>GSHMKNSVSVDLPGSMKVLVSKSSNADGKYDLIATVDALELSGTSDKNNGSGVLEGVKADASKVKLTISDDLGQTTLEVFKSDGSTLVSKKVTSKDKSSTYELFNEKGELSFKYITRADKSSTYELFNEKGELSFKYITRADKSSTYELFNEKGELSFKYITRADKSSTYELFNEKGELSFKYITRADGTRLEYTGIKSDGSGKAKEVLKGYVLEGTLTAEKTTLVVKEGTVTLSKNISKSGEVSVELNDTDSSAAT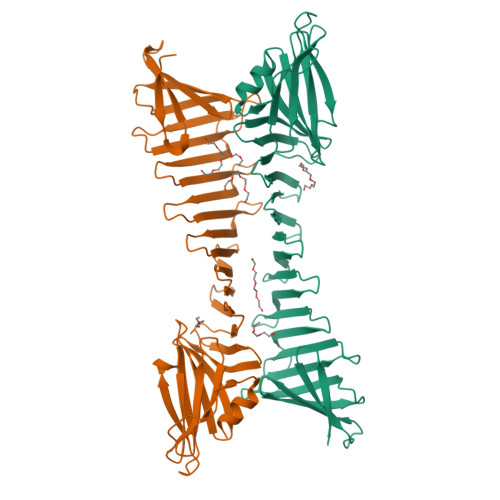KKTAAWNSGTSTLTITVNSKKTKDLVFTSSNTITVQQYDSNGTSLEGSAVEITKLDEIKNALK[2x]N~3~-phenyl-1-[6-(phenylamino)pyrimidin-4-yl]-1H-1,2,4-triazole-3,5-diamine | C18 H16 N8 | 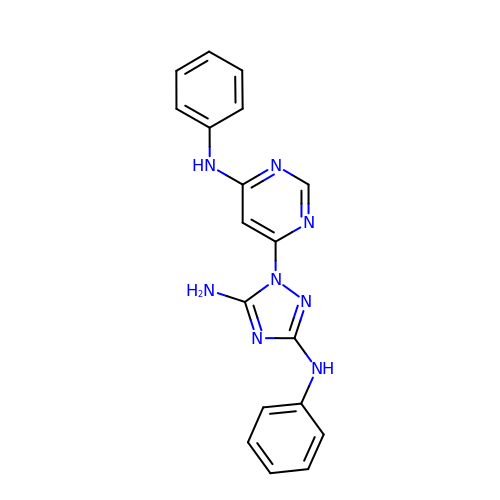PYFLNUFSEAXOHE-UHFFFAOYSA-N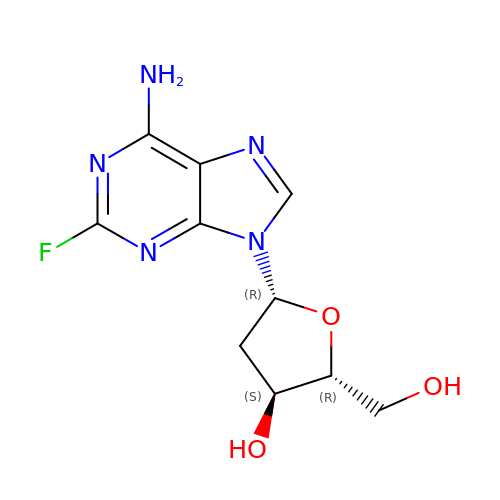5-(6-AMINO-2-FLUORO-PURIN-9-YL)-2-HYDROXYMETHYL-TETRAHYDRO-FURAN-3-OL | C10 H12 F N5 O3 | ZWPYUXAXLRFWQC-KVQBGUIXSA-N> MDEKLLKTIAESKYLVALTGAGVSAESGIPTFRGKDGLWNRYRPEELANPQAFAKDPEKVWKWYAWRMEKVFNAQPNKAHQAFAELERLGVLKCLITQNVDDLHERAGSRNVIHLHGSLRVVRCTSCNNSFEVESAPKIPPLPKCDKCGSLLRPGVVWFGEML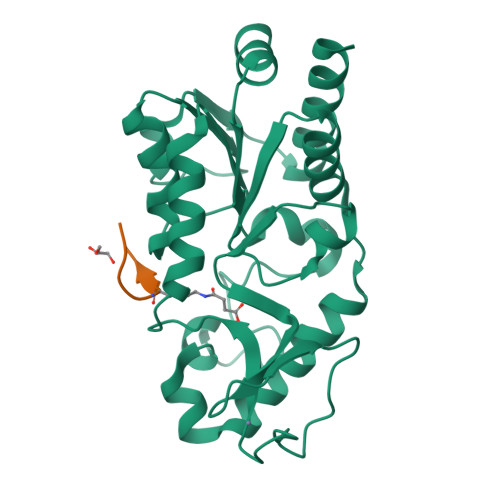PPDVLDRAMREVERADVIIVAGTSAVVQPAASLPLIVKQRGGAIIEINPDETPLTPIADYSLRGKAGEVMDELVRHVRKALS;> KGLGKGGAXRHRKW> MAEPGIDKLFGMVDSKYRLTVVVAKRAQQLLRHGFKNTV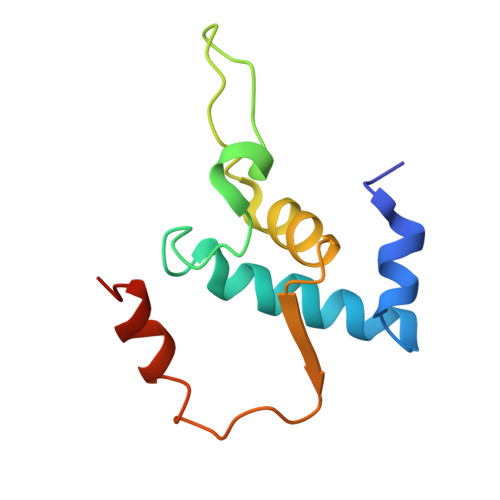LEPEERPKMQTLEGLFDDPNAETWAMKELLTGRLVFGENLVPEDRLQKEMERIYPGEREE Glutamine synthetases (GS) catalyze the ATP-dependent ammonium assimilation, the initial step of nitrogen acquisition that must be under tight control to fit cellular needs. The dodecamer is organized as two stacked hexameric rings, and each polypeptide is organized into two parts, a shorter N-terminal domain (β-Grasp fold) and the remaining C-terminal domain. The active sites are located at the interface of the N- and C- terminal domains of the adjacent subunit in the hexameric ring. Two loops in the active center are critical for catalysis: the Glu-flap, involved in shielding the active site during catalysis and deprotonating the intermediate product, and the Asp-50’ loop, which binds and deprotonates ammonium.

The complex with 2OG/Mg2+ was obtained with and without ATP (MtGS-2OG/Mg2+/ATP, MtGS-2OG/Mg2+) in a new crystalline form and both were refined to 2.15 Å and 2.91 Å resolution, respectively. Both 2OG-containing structures show high tridimensional conservation (rmsd 0.279 Å, 441 atoms aligned) while deviating from the apo resting state (2OG/Mg2+/ATP:rmsd 0.694 Å, 374 atoms aligned, 2OG/Mg2+: 0.631 Å, 371 atoms aligned). The structure of MtGS reveals an allosteric pocket perfectly suited to accommodate 2OG via specific salt bridges, hydrogen bonds, and Van der Waals contacts. Binding of 2OG leads to a succession of conformational rearrangements resulting in a catalytically competent state. The repositioning of the N-terminal domain would clash with the next monomer, and therefore a domino effect occurs in the hexamer ring upon 2OG binding. Overall, the transition between MtGS resting and 2OG-bound states provokes a compaction of the outer ring and an opening in the center and middle parts, leading to a more “opened” conformation. In MtGS the 2OG binding provokes a major displacement of the N-terminal domain towards the adjacent C-terminal domain and the overall conformational changes promote a restructuration of the Asp50ʹ-loop, leading to the repositioning of Arg321 and the Glu-flap, yielding an active conformation.

>[24x]MSTVEQVLEYVKSNNVKFMRFQFVDILGVPKNVAFPIKAGEKGIEELRDVLENGLYFDGSSIEGFVGINESDMMLKPDLSTFSVLPWRPSEKSVARVICDVYTTKGKPFEGDPRGCLKRVMEEFKKEFNGEYFVGPEPEFFLLKKDPHNPHKYIPADDGGYFDLEPMDEAPDIRRDIVFALENLGFHVEASHHEVAPGQHEVDFKFDDALKTADSVITFKTTIKTIAEQHGLKATFMPKPFFGMNGSGMHCHQSIWLNGEPSFYDENAPYQLSETCMNYVAGILKHAKAIVAITNPTVNSYKRLVPGYEAPVNIAWANSNRSAIIRVPAARGKGTRIEFRAPDPSCNPYLAFTVMLAAGLDGVKNKLDAPEPVERNIFAMSEAEKKELGIESVPANLKAALDELENNDVLKNALGKHIFESFLEIKNAEWDSFRTSVTDWETTAYLKI tert-butyl [(2-amino-4-oxo-4,7-dihydro-3H-pyrrolo[2,3-d]pyrimidin-5-yl)methyl]carbamate 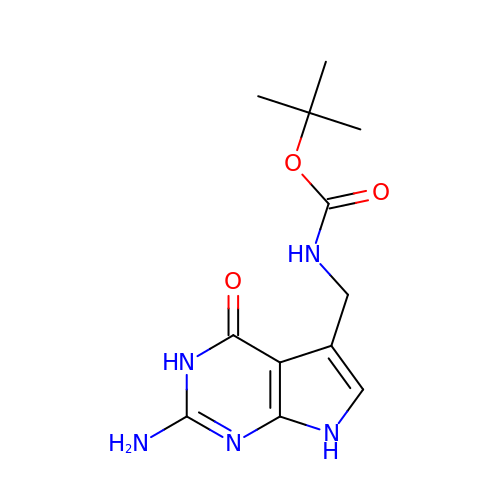| C12 H17 N5 O3 | RXVQMCMIOHBKNE-UHFFFAOYSA-N>[2x]GPLGSMEGFERELDNIPDTLPDDERLALWKGKLKHYLILSSAGKPIWSRHGDLSLVNSTMGVVQTIISFYEGARNPLLGFTAGKVRFVILIKGPLYFVAISRLRESDAQLRAQLEALYMQILSTLTLPILTNIFAHRPSTDLRGPLQGTESLLASLADSFTKGSPS;>SMTTPVSPSPSGIIPAQLGFLAIYNPALGTTDETLEDQIVYYATASTLSQARRRHRRPRRRDRQRAQSVVKDSRPNAAGATGDSEAVAEDKDPVSKEERHERLRQIGLAQGMVEFAKSFSDGEPVDTIDTEKARVILVEVEEGWWILASIDLTRLPLPQIKTPTSSSAPPPAPNLNPLPPEPAYEYSSREVKPPSLLRADLLR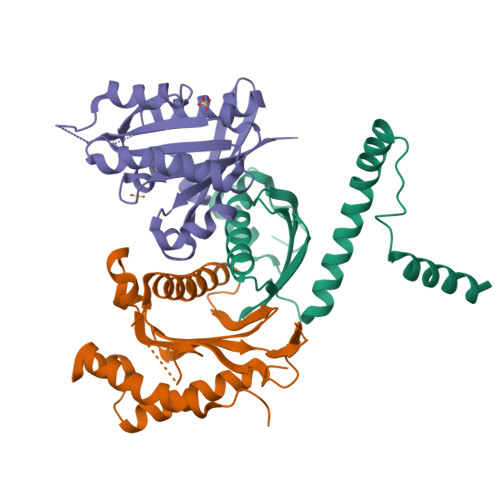AYDLFLLHHGSSLSSLLASQGRAQLVASLTRFWDHFLATWNVLLHGN[2x];>[2x]GSMSSRKKVLLKVIILGDSGVGKTSLMNQYVNKKFSASYKATIGADFLTREVMVDDRQVTMQLWDTAGQERFQSLGVAFYRGADCCVLVFDVNNAKSFDALDSWRDEFLIQASPRDPENFPFVVLGIKIDVEESKRVISTKRAQTFCQSKGGIPYFETSAKEAINVEEAFQVIARNALMQEESEEFSGDFQDPINIHIENERDGCAC Ribonuclease A was one of the first enzymes to be studied by X-ray crystallography. The commonly accepted residues associated with the active site of Bovine RNase A are Lys 7, Gln 11, His 12, Lys 41, Asn 44 and His 119. Waters W86 and W91 make interactions with imidazole groups of His-105 and His-119, respectively. Both His-119 and His-12 are known to be involved in the catalytic mechanism for cyclization and cleavage of RNA. The crystal structure of orthorhombic Bovine Pancreatic Ribonuclease A has been determined to 0.85 Å resolution using low temperature, 100 K, synchrotron X-ray data collected at 16000 keV (λ = 0.77 Å). This is the first ultra-high-resolution structure of a native form of Ribonuclease A to be reported.

The space group is: P212121 (19) and the unit cell is: a = 43.9980 Å, b = 45.6970 Å, c = 51.8900 Å, α = 90°, β = 90o, γ = 90°. Refinement carried out with anisotropic displacement parameters, stereochemical restraints, inclusion of H atoms in calculated positions, five SO42- moieties, eleven ethanol molecules and 293 water molecules, converged with final R values of R1(Free) = 0.129 (4279 reflections) and R1 = 0.112 (85,346 reflections). Five SO42- moieties and eleven ethanol molecules were located and refined in the 0.85Å Orthorhombic RNase A structure designated SO41151 to1155 and EOH A201 to A211, respectively. In the orthorhombic structure Lys-7, Gln-11, His-12, Asn-44 and His-119 occupy single sites while Lys-41 is disordered into sites A and B and the SO42- group into sites A (60%) and B (40%). The A site hydrogen bonds to His-12, and Gln-11 while the B-site hydrogen bonds to Gln-11, His-119 and a water molecule. In Orthorhombic RNase His-12 H-bonds to the SO42- group both directly and via a water molecule. There is good clear electron density for this residue which has been modelled largely as a single conformation but with a minor branch at the end.

> KETAAAKFERQHMDSSTSAASSSNYCNQMMKSRNLTKDRCKPVNTFVHESLADVQAVCSQKNVACKNGQTNCYQSYSTMSITDCRETGSSKYPNCAYKTTQANKHIIVACEGNPYVPVHFDASV>ETGGLLNCPIYWQQLREKCLLFSHTVNPWNNSLADCSTKES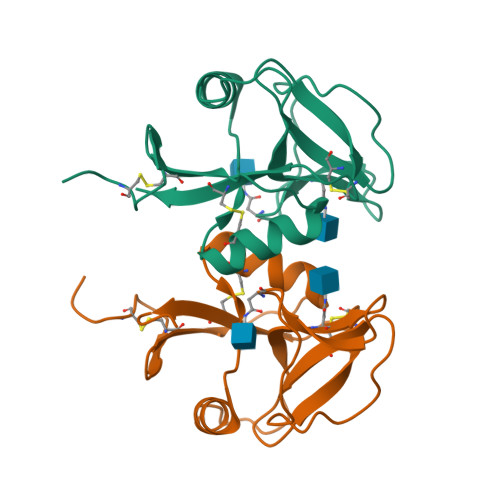SLLLIRDKDELIHTQNLIRDKAILFWIGLNFSLSEKNWKWINGSFLNSNDLEIRGDAKENSCISISQTSVYSEYCSTEIRWICQKELTPVRNKVYPDSKHHHHHH[8x]> MSELERHSYDVVVIGAGGAGLRAVI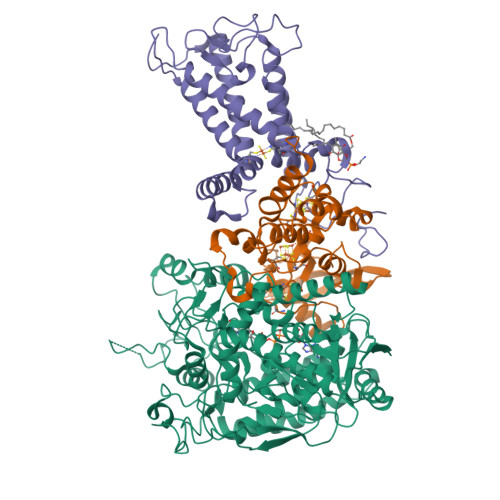EARERGLRVAVVTKSLFGKAHTVMAEGGCAAAMRNVNTKDSWQVHFGDTMRGGKFLNNWRMAELHAQEAPDRVWELETYGALFDRTKDGKISQRNFGGHTYPRLAHVGDRTGLEIIRTLQQKIVSLQQEDKRELGDYEARIRVFHETSITELILDDGKIAGAFGYYRETGNFVLFEAPAVVLATGGIGKSFKVSSNSWEYTGDGHALALRAGSALINMEFIQFHPTGMVWPLSVKGILVTEGVRGDGGVLKNSEGKRFMFDYIPSVFKGQYAETEEEADQWLKDNDSARRTPDLLPRDEVARAINAEVKAGRGSPHGGVYLDIASRMPAEEIKRRLPSMYHQFIELAEVDITKDAMEVGPTCHYVMGGIEVDPDTAAGATPGLFAAGECSGGMHGSNRLGGNSLSDLLVFGRRAGLGAADYVRALPDRPKVSEAAVEDATRLVLAPFEPKAEPENPYTLHAELQQSMNDLVGIIRKEAEIQEALDRLQELKRRYANVTVEGGRVFNPGWHLAIDMRNMLLVSECVAKAALQRTESRGGHTRDDYPEMDANWRNTLLVCRVSGGDPVVPDVTVTPEQQVPMRPDLLGCFELSELEKYYTPEELAEHPERKG;> MATYDAKLRVWRGDDTGGELHDYTVEVNDGEVVLDIIHRLQATQTPDLAVRWNCKAGKCGSCSAEINGRPRLMCMTRMSTFGEDEVVTVTPLRTFPVMRDLVTDVSFNYEKARQIPSFTPPKDLQPGEYRMQQEDVNRSQEFRKCIECFLCQNVCHVVRDHEENKENFAGPRFHMRIAELDMHPLDTVDRKEMAQDEFGLGYCNITKCCTEVCPEHIKITDNALIPMKERVADRKYDPIVWLGNKLFRR;> MSAPTADRRATGVFSPRRAQIPERTLRTDRWWQAPLLTNLGLAAFVIYATIRAFWGSAYWVADYHYLTPFYSPCVSTACAPGSSHFGQWVGDLPWFIPMAFISLPFLLAFRLTCYYYRKAYYRSVWQSPTACAVAEPHAKYTGETRFPLILQNIHRYFFYAAVLISLVNTYDAITAFHSPSGFGFGLGNVILTGNVILLWVYTLSCHSCRHVTGGRLKHFSKHPVRYWIWTQVSKLNTRHMLFAWITLGTLVLTDFYIMLVASGTISDLRFIGHHHHHHHHHH> QEDEDGDYE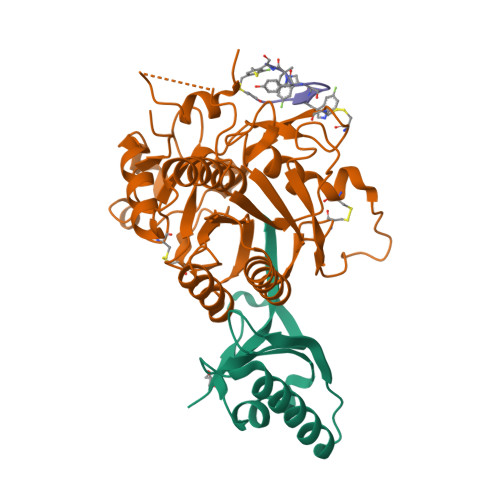ELVLALRSEEDGLAEAPEHGTTATFHRCAKDPWRLPGTYVVVLKEETHLSQSERTARRLQAQAARRGYLTKILHVFHGLLPGFLVKMSGDLLELALKLPHVDYIEEDSSVFAQ;> SIPWNLERITPPRYRADEYQPPDGGSLVEVYLLDTSIQSDHREIEGRVMVTDFENVPEEDGTRFHRQASKCDSHGTHLAGVVSGRDAGVAKGASMRSLRVLNCQGKGTVSGTLIGLEFIRKSQLVQPVGPLVVLLPLAGGYSRVLNAACQRLARAGVVLVTAAGNFRDDACLYSPASAPEVITVGATNAQDQPVTLGTLGTNFGRCVDLFAPGEDIIGASSDCSTCFVSQSGTSQAAAHVAGIAAMMLSAEPELTLAELRQRLIHFSAKDVINEAWFPEDQRVLTPNLVAALPPSTHGAGNSHHHHHH;> CKAWWPTYXCA>SMKLDIKKTFSNRSDRVAGIDFHPTEPWVLTTLYSGRVEIWNYETQVEVRSIQVTETPVRAGKFIARKNWIIVGSDDFRIRVFNYNTGEKVVDFEAHPDYIRSIAVHPTKPYVLSGSDDLTVKLWNWENNWALEQTFEGHEHFVMCVAFNPKDPSTFASGCLDRTVKVWSLGQSTPNFTLTTGQERGVNYVDYYPLPDKPYMITASDDLTIKIWDYQTKSCVATLEGHMSNVSFAVFHPTLPIIISGSEDGTLKIWNSSTYKVEKTLNVGLERSWCIATHPTGRKNYIASGFDNGFTVLSLG[2x]

Hence, this loss of critical proteins has the potential to compromise ER proteostasis and generate cellular stress. This challenge to normal metabolism is overcome by the activity of the cytosolic coatomer protein I (COPI) polymer, whose repeating unit is the coatomer, a 560 kDa complex of seven distinct gene products (α-, β-, β′-, γ-, δ-, ε-, and ζ-COPI)25–31. Overall, the coatomer functions to retrieve the escaped “client” proteins, such as type I membrane proteins, from cis-Golgi back to ER by retrograde trafficking. In particular, the S protein – a type I membrane protein – is delivered to the ERGIC from both the ER (by anterograde trafficking) and the Golgi (by retrograde trafficking)3,10–12. Here we utilize recombinant SARS-CoV-2 S proteins and tail peptides, including constructs with enhanced mimicry of the coatomer binding motif (clientized S protein), to elucidate the atomic structure of the S-coatomer interface.

We hypothesized that if the interaction site is comparable between the αWD40 and β‘WD40 domains, then a disruptive substitution at a juxtaposed critical WD40 residue should yield a similar weakening of S tail interaction with either domain. Therefore, we expressed and purified an alanine substitution mutant of β‘WD40 Lys17, which is juxtaposed with αWD40 Lys15. This β‘WD40 mutant demonstrated a lack of binding to the clientized Thr1273Glu S tail heptapeptide, which is consistent with the loss of binding displayed by the αWD40 Lys15Ala mutant. Next, we determined a 2 Å resolution crystal structure of this domain. This showed a rotation of the Arg15 side-chain reminiscent of the conformational change reported above in the αWD40 Lys15Ala mutant.>[2x]MAHHHHHHMTHALFTKHEDTLKRALAAIESRGYWSPFAEMPSPKVYGESGNADGEAAFKSHLGKTFELDQPASGETVGAERSPYGVALDIRYPKSTPDALIAAAAAAQRTWREAGPSAWIGVSLEILARLNRASFEIAYSVMHTTGQAFMMAFQAGGPHAQDRALEAVAYAWDQLRRIPADAHWEKPQGKNPPLAMQKRYTIVPRGTGLVLGCCTFPTWNGYPGLFADLATGNTVIVKPHPGAILPLAITVRIARDVLREAGFDPNVVTLLATEPNDGALVQDLALRPEIKLIDFTGSTQNGTWLERHAHQAQVYTEKAGVNQIVIDSTDDLKAAAKNIAFSLALYSGQMCTAPQNIYVPRDGIRTADGHASFDEVAQAIAGAVQKLTGDPARSVE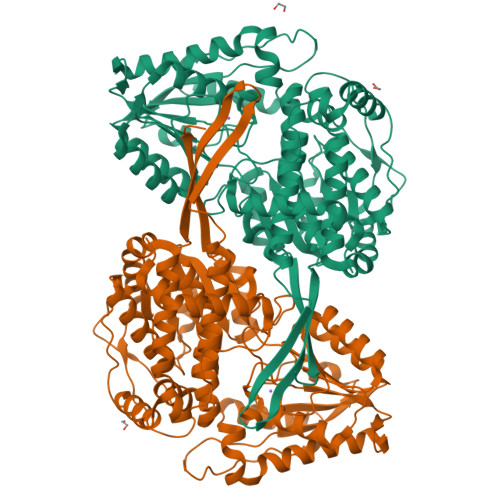LIGAIQNDGVTARIDAARAVGRVLLDSQTLQHPAFPDARVRTPLVLQLDVADREKFTQEWFGPISFVIATDSTAQSLDLAGEIAAEHGALTLSVYSTADDVIDAAHEAAVRGGVALSINLTGGVFVNQSAAFSDFHGTGANPAANAALADAAFVANRFRVVQSRVHVAPKAAPAEVGQPA>[3x]MSDNNDRMYELEYPSPEVSGQTAGGPTLIVALQGYADAGHAVESSSSHLMDALDHRLIASFNNDELIDYRSRRPVVVIEHNEVTSMDELNLGLHVVRDNDNKPFLMLSGPEPDLRWGDFSNAVVDLVEKFGVENTICLYAAPMTVPHTRPTVVTAHGNSTDRLKDQVSLDTRMTVPGSASLMLEKLLKDKGKNVSGYTVHVPHYVSASPYPAATLKLLQSIADSAD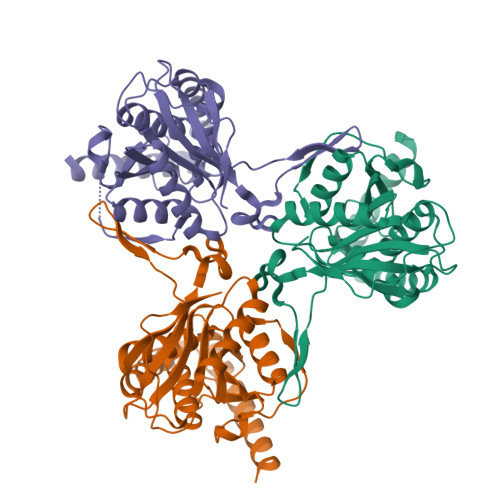LNLPLLALERDAEKVHRQLMEQTEESSEIQRVVGALEQQYDSELERYRNRHPQAVMPGESELPSGDEIGAEFEKFLADLDDQGGSDHKETPEA> MKKVVAVVKLQLPAGKATPAPPVGPALGQHGANIMEFVAAFNAATANMGDAIVPVEITIYADRSFTFVTKTPPASYLIRKAAGLEKGAHKPGREKVGRITWEQVLEIAKQKMPDLNTTDLEAAARMIAGS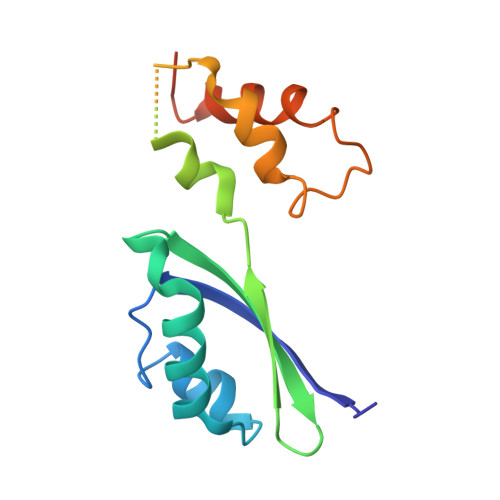ARSMGVEVVGAPEVKDA>[2x]MS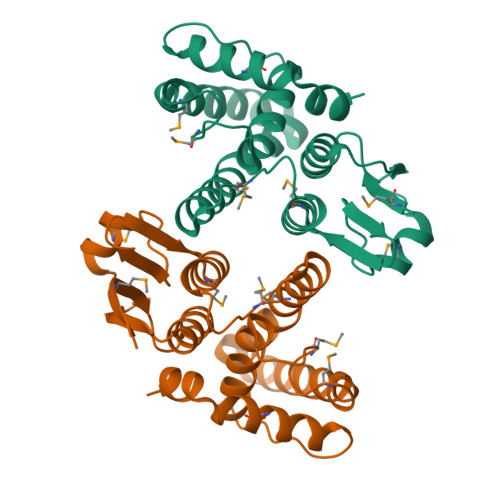LRSVMTLFSNKDDIYCHQVKIVLAEKGVLYENAEVDLQALPEDLMELNPYGTVPTLVDRDLVLFNSRIIMEYLDERFPHPPLMQVYPVSRAKDRLLMLRIEQDWYPTLAKAENGTEKEKTSALKQLKEELLGIAPIFQQMPYFMNEEFGLVDCYVAPLLWKLKHLGVEFTGTGSKAIKAYMERVFTRDSFLQSVGEAAPKNLMDDKEGHHHHHH> MEPIEEATKCYDQMLIVERYERVISYLYPIAQSIPRKHGVAREMFLKCLLGQVELFIVAGK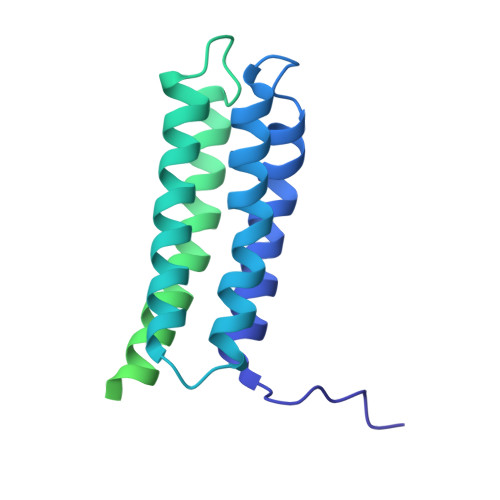SNQVSKLYAADAGLAMLRFWLRFLAGIQKPHAMTPHQVETAQVLIAEVGRILGSWIARVNRKGTKVQVGEALVGDGNEVAHIDLIIGPRGSPAETAFCNGLVNNKHGFTSLLAVIAPNLPCKPNTLMFNKVTINDARQAVQMFGPAQHGVAMAVQDAVAEGIIPADEADDLYVLVGVFIHWEAADDAKIQKYNYEATKLSIQRAVNGEPKASVVTEQRKSATHPFAANA>NNPSAAVVVSSRWNPTPEQLRALEELYRRGTRTPSAEQIQQITAQLRKFGKIEGKNVFYWFQNHKARERQKRRRQMESAAAEFDSAIEKKDLGASRTVFEVEHTKN[2x]

In plants, the WUSCHEL-related homeobox (WOX) family of transcription factors function as central organizers of several developmental programs ranging from embryo patterning to meristematic stem-cell maintenance through transcriptional activation and repression mechanisms. The Medicago truncatula STENOFOLIA (STF) gene is a master regulator of leaf-blade lateral development. The Medicago truncatula WOX1 gene, STENOFOLIA (STF), and its Nicotiana sylvestris ortholog, LAMINA1 (LAM1), regulate leaf-blade outgrowth by promoting cell proliferation at the adaxial–abaxial junction through transcriptional repression. While the HD contacts DNA, the WUS box is essential for the recruitment of the TOPLESS (TPL) family of transcriptional co-repressors.

Here, the crystal structure of the homeodomain (HD) of STF (STF-HD) in complex with its promoter DNA is reported at 2.1 Å resolution. The structure of the complex was determined by single-wavelength anomalous dispersion using a SeMet-substituted crystal of the triple-mutant STF protein (L107M/L110M/L130M; see Section 2). There are two protein molecules and one DNA molecule in the asymmetric unit of the crystal. The overall structure of STF-HD adopts the canonical HD architecture comprised of a three-α-helical bundle core connected by well ordered loops and a long arm of peptide at the N-terminus, with overall dimensions of approximately 42 × 32 × 25 Å. The two protomers HDA and HDB are positioned more than 8 Å apart and are bound on the opposite sides of the DNA, making no direct protein–protein interactions with each other. There are also two additional STF-HD molecules bound on the same DNA (HDA′ and HDB′), which are related to HDA and HDB, respectively, in the crystal via crystallographic symmetry, forming a tetramer. The STF-HD tetramer interacts with the DNA extensively. HDA and HDB are bound at two TGA motifs that are arranged as an inverted repeat and are separated by five base pairs, making contacts with the DNA via both the major and minor grooves. In both HDA and HDB, the N-terminal arms embrace the DNA from the minor grooves, while the α3 helices are inserted into the major grooves of the DNA. Arg96 (N-terminal arm), Asn147 and Arg151 (helix α3) serve as a molecular probe for STF to read out the TGA DNA fingerprint. The two crystallographic symmetry-related STF-HD molecules, HDA′ and HDB′, mainly contact the DNA in the minor grooves using polar and basic residues located in the C-terminal halves of their α3 helices.>GAAAAMSICPHIQQVFQNEKSKDGVLKTCNAARYILNHSVPKEKFLNTMKCGTCHEINSGATFMCLQCGFCGCWNHSHFLSHSKQIGHIFGINSNNGLLFCFKCEDYIGNIDLINDAILAKYWDDVCTKTMVPSMERRDGLSGLINMGSTCFMSSILQCLIHNPYFIRHSMSQIHSNNCKVRSPDKCFSCALDKIVHELYGALNTKQASSSSTSTNRQTGFIYLLTCAWKINQNLAGYSQQDAHEFWQFIINQIHQSYVLDLPNAKEVSRANNKQCECIVHTVFEGSLESSIVCPGCQNNSKTTIDPFLDLSLDIKDKKKLYECLDSFHKKEQLKDFNYHCGECNSTQDAIKQLGIHKLPSVLVLQLKRFEHLLNGSNRKLDDFIEFPTYLNMKNYCSTKEKDKHSENGKVPDIIYELIGIVSHKGTVNEGHYIAFCKISGGQWFKFNDSMVSSISQEEVLKEQAYLLFYTIRQVN[2x];>[2x]MTMDTAQLK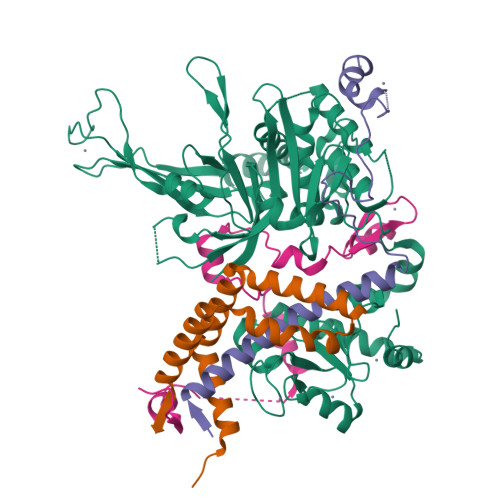SQIQQYLVESGNYELISNELKARLLQEGWVDKVKDLTKSEMNINESTNFTQILSTVEPKALEMVSDSTRETVLKQIREFLEEIVDTQ;>MTEETITIDSISNGILNNLLTTLIQDIVARETTQQQLLKTRYPDLRSYYFDPNGSLDINGLQKQQESSQYIHCENCGRDVSANRLAAHLQRCLSRGARR[2x];>[2x]MRSGDAEIKGIKPKVIEEYSLSQGSGPSNDSWKSLMSSAKDTPLQYDHMNRESLKKYFDPNAQLIEDPLDKPIQYRVCEKCGKPLALTAIVDHLEN>MEHHHHHHATNLRGVMAALLTPFDQQQALDKASLRRLVQFNIQQGIDGLYVGGSTGEAFVQSLSEREQVLEIVAEEAKGKIKLIAHVGCVSTAESQQLAASAKRYGFDAVSAVTPFYYPFSFEEHCDHYRAIIDSADGLPMVVYNIPALSGVKLTLDQINTLVTLPGVGALKQTSGDLYQMEQIRREHPDLVLYNGYDNIFASGLLAGADGGIGSTYNIMGWRYQGIVKALKEGDIQTAQKLQTECNKVIDLLIKTGVFRGLKTVLHYM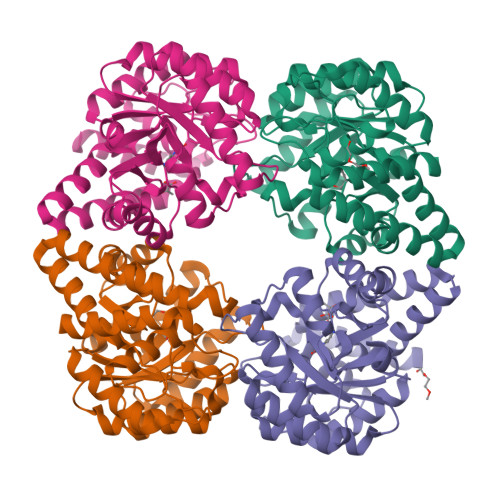DVVSVPLCRKPFGPVDEKYLPELKALAQQLMQER[4x]>MAHHHHHHVTNSTDGRADGRLRVVVLGSTGSIGTQALQVIADNPDRFEVVGLAAGGAHLDTLLRQRAQTGVTNIAVADEHAAQRVGDIPYHGSDAATRLVEQTEADVVLNALVGALGLRPTLAALKTGARLALANKESLVAGGSLVLRAARPGQIVPVDSEHSALAQCLRGGTPDEVAKLVLTASGGPFRGWSAADLEHVTPEQAGAHPTWSMGPMNTLNSASLVNKGLEVIETHLLFGIPYDRIDVVVHPQSIIHSMVT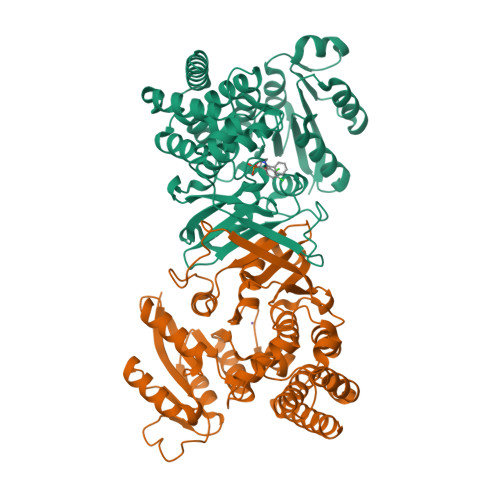FIDGSTIAQASPPDMKLPISLALGWPRRVSGAAAACDFHTASSWEFEPLDTDVFPAVELARQAGVAGGCMTAVYNAANEEAAAAFLAGRIGFPAIVGIIADVLHAADQWAVEPATVDDVLDAQRWARERAQRAVSGM[2x]>[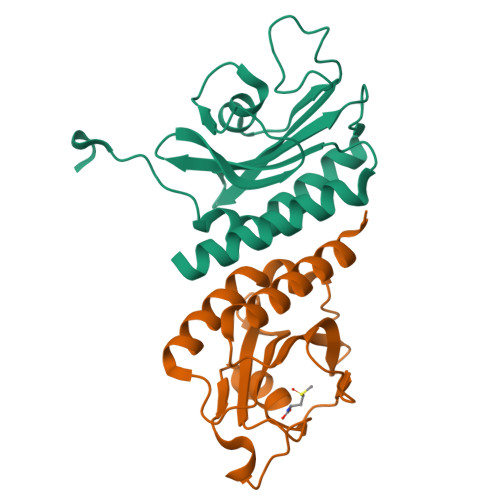2x]MDLKEFARSQMQAACQYLKEKNPKYDWVGFYVLEHGKLKLEAFVGEKTDHVEINLGDGLCSLAVLKNDIVNEYDVKSNPKYLASFPSTQSEIVVPVRYQGEPIGEIDIDSDKKAAFSKEDEAMLSSIADLMAPLVHEFFVKLEHHHHHH>SGGGMLTLIQGKKIVNHLRSRLAFEYNGQLIKILSKNIVAVGSLRREEKMLNDVDLLIIVPEKKLLKHVLPNIRIKGLSFSVKVCGERKCVLFIEWEKKTYQLDLFTALAEEKPYAIFFFTGPVSYLIRIRAALKKKNYKLNQYGLFKNQTLVPLKITTEKELIKELGF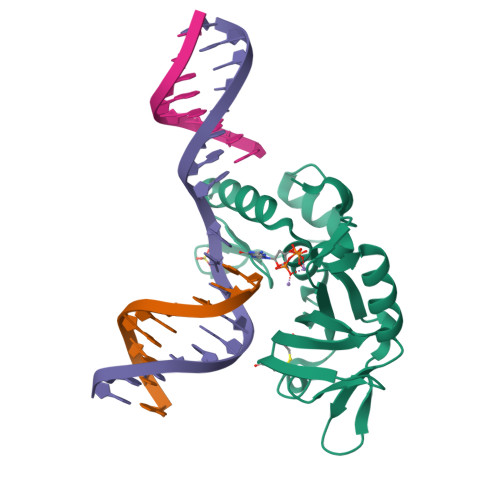TYRIPKKRL[2x]> PPGTVDKKMVEKCWKLMDKVVRLCQNPKLALKNSPPYILDLLPDTYQHLRTILSRYEGKMETLGENEYFRVFMENLMKKTKQTISL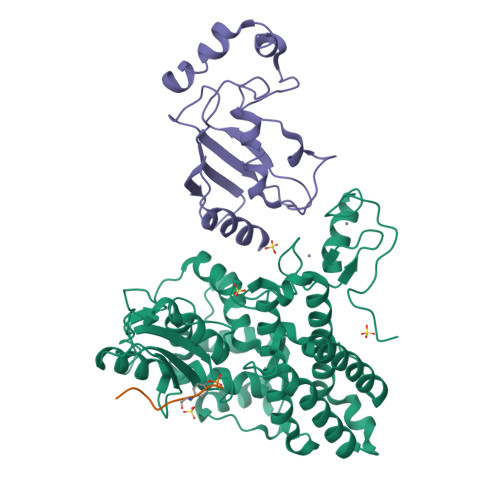FKEGKERMYEENSQPRRNLTKLSLIFSHMLAELKGIFPSGLFQGDTFRITKADAAEFWRKAFGEKTIVPWKSFRQALHEVHPISSGLEAMALKSTIDLTCNDYISVFEFDIFTRLFQPWSSLLRNWNSLAVTHPGYMAFLTYDEVKARLQKFIHKPGSYIFRLSCTRLGQWAIGYVTADGNILQTIPHNKPLFQALIDGFREGFYLFPDGRNQNPDLTGLCEPTPQDHIKVTQEQYELYCEMGSTFQLCKICAENDKDVKIEPCGHLMCTSCLTSWQESEGQGCPFCRCEIKGTEPIVVDPF;> SDGYTPEPA;> MAASRRLMKELEEIRKCGMKNFRNIQVDEANLLTWQGLIVPDNPPYDKGAFRIEINFPAEYPFKPPKITFKTKIYHPNIDEKGQVCLPVISAENWKPATKTDQVIQSLIALVNDPQPEHPLRADLAEEYSKDRKKFCKNAEEFTKKYGEKRPVD> ILGGTEAEEGSWPWQVSLRLNNAHHCGGSLINNMWILTAAHCFRSNSNPRDWIATSGISTTFPKLRMRVRNILIHNNYKSATHENDIALVRLENSVTFTKDIHSVCLPAATQNIPPGSTAYVTGWGAQEYAGHTVPELRQGQVRIISNDVCNAPHSYNGAILSGMLCAGVPQGGVDACQGDAGGPLVQEDSRRLWFIVGIVSWGDQCGLPDKPGVYTRVTAYLDWIR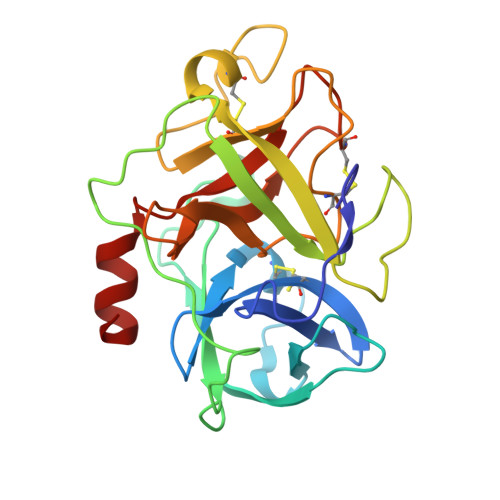QQTGI> MTQETTTLTGQSPPPVRDWPALDLDGPEFDPVLAELMREGPLTRVRLPHGEGWAWLATRYDDVKAITNDPRFGRAEVTQRQITRLAPHFKPRPGSLAFADQPDHNRLRRAVAGAFTVGATKRLRPRAQEILDGLVDGIL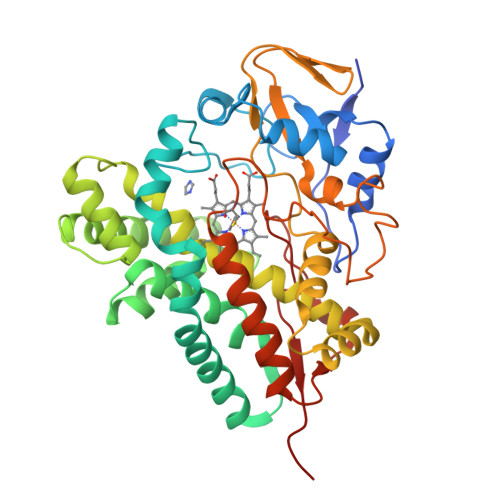AEGPPADLVERVLEPFPIAVVSEVMGVPAADRERVHSWTRQIISTSGGAEAAERAKRGLYGWITETVRARAGSEGGDVYSMLGAAVGRGEVGETEAVGLAGPLQIGGEAVTHNVGQMLYLLLTRRELMARMRERPGARGTALDELLRWISHRTSVGLARIALEDVEVHGTRIAAGEPVYVSYLAANRDPDVFPDPDRIDLDRDPNPHLAYGNGHHFCTGAVLARMQTELLVDTLLERLPGLRLAVPAEQVAWRRKTMIRGPRTLPCTWHHHH> MHLMRACITFCIASTAVVAVNAALVAEDAPVLSKAFVDRVNRLNRGIWKAKYDGVMQNITLREAKRLNGVIKKNNNASILPKRRFTEEEACAPLPSSFDSAEAWPNCPTIPQIADQSACGSCWAVAAASAMSDRFCTMGGVQDVHISAGDLLACCSDCGDGCNGGDPDRAWAYFSSTGLVSDYCQPYPFPHCSHHSKSKNGYPPCSQFNFDTPKCNYTCDDPCIPVVNYRSWTSYALQGEDDYMRELFFRGPFEVAFDVYEDFIAYNSGVYHHVSGQYLGGHAVRLVGWGTSNGVPYWKIANSWNTEWGMDG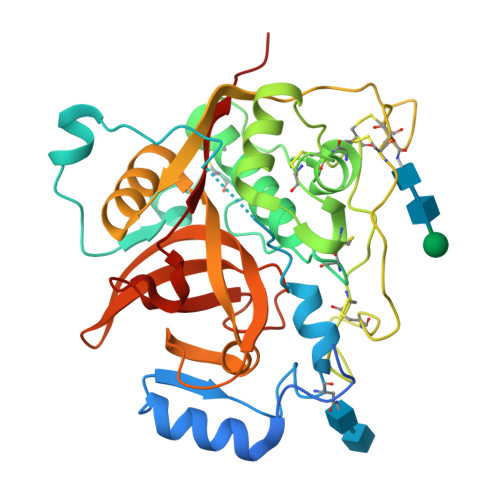YFLIRRGSSECGIEDGGSAGIPLAPNTA>MNRLPYFINYFFDTYLLINEDTPVGSSVTQLLARDLDNDHLV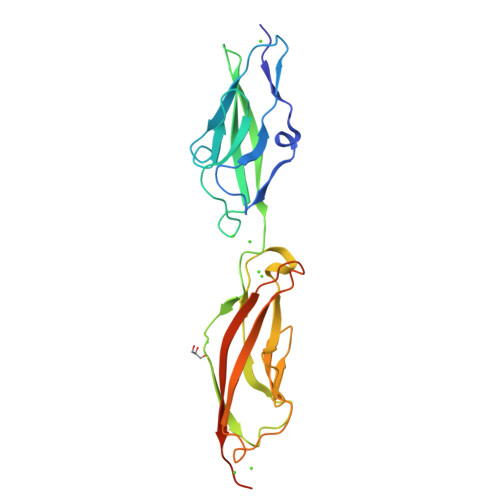FGVVGEEASRFFAVESVTGVVWLRQPLDRETKSEFTVEFSVSDSQGVIKGTVNIQVGDVNDNAPRFHNQPYSVRIAENTPVGTPIFIVNATDPDQGAGGSVLYSFQPPSSFFAIDSGRGIVSVIRGLDYEITQAYQLQVNATDQDKSKPLSTLANLAITITDVQDMDPLEHHHHHH[4x]>SCGCFEAIMAILPECNGIMITTRDHAGMTPSGMTFSTLAGMIGGGTQTPGFMGIGRTYIVSKKFISADGGIARIVWMPKS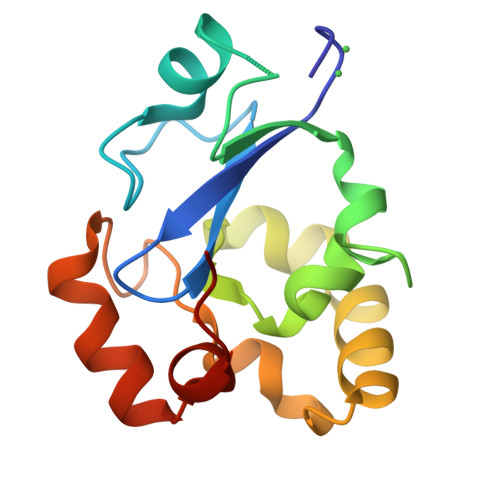LKDFLHDEFVRRSVEEGLGEDFIDKIADETIGTTVDEILPYLEEKGHPALTMDPIMA[2x]4-{[(2S)-2-butyl-6,7-dichloro-2-cyclopentyl-1-oxo-2,3-dihydro-1H-inden-5-yl]oxy}butanoic acid | C22 H28 Cl2 O4 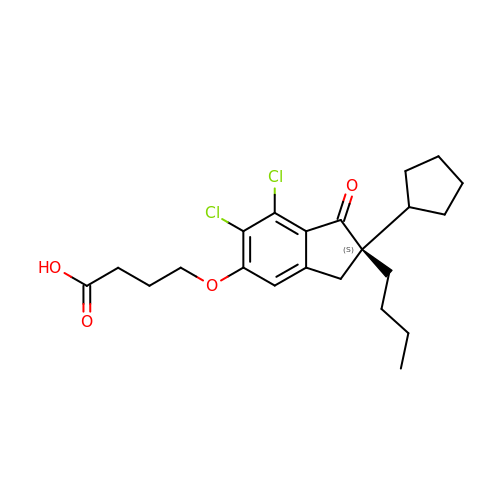| KHKGTPJPBOQECW-QFIPXVFZSA-N3-methyl-2-(prop-2-ynoxymethyl)imidazol-4-amine 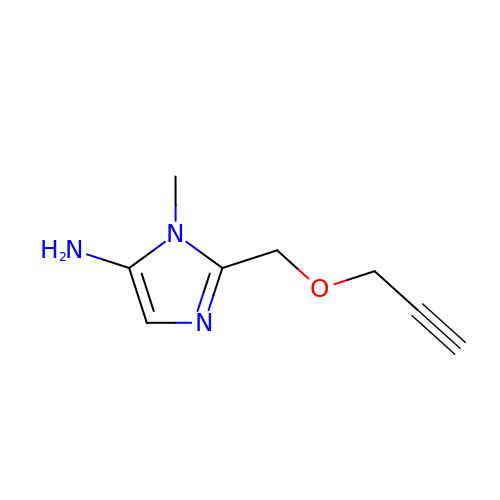| C8 H11 N3 O | JGQPVNNBPSNUGF-UHFFFAOYSA-N N,N'-Bis(3-aminopropyl)-1,4-cyclohexanediamine | C12 H28 N4 | 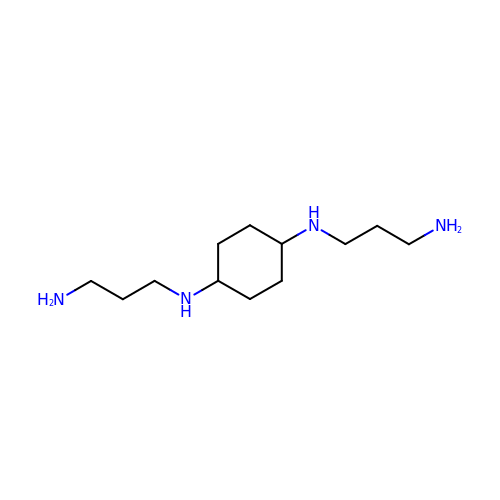PYBOSIQOXDJMFB-HAQNSBGRSA-N> MPYSVGFREADAATSFLRAARSGNLDKALDHLRNGVDINTCNQNGLNGLHLASKEGHVKMVVELLHKEIILETTTKKGNTALHIAALAGQDEVVRELVNYGANVNAQSQKGFTPLYMAAQENHLEVVKFLLENGANQNVATEDGFTPLAVALQQGHENVVAHLINYGTKGKVRLPALHIAARNDDTRTAAVLLQNDPNPDVLSKTGFTPLHIAAHYENLNVAQLLLNRGASVNFTPQNGITPLHIASRRGNVIMVRLLLDRGAQIETKTKDELTPLHCAARNGHVRISEILLDHGAPIQAKTKNGLSPIHMAAQGDHLDCVRLLLQYDAEIDDITLDHLTPLHVAAHCGHHRVAKVLLDKGAKPNSRALNGFTPLHIACKKNHVRVMELLLKTGASIDAVTESGLTPLHVASFMGHLPIVKNLLQRGASPNVSNVKVETPLHMAARAGHTEVAKYLLQNKAKVNAKAKDDQTPLHCAARIGHTNMVKLLLENNANPNLATTAGHTPLHIAAREGHVETVLALLEKEASQACMTKKGFTPLHVAAKYGKVRVAELLLERDAHPNAAGKNGLTPLHVAVHHNNLDIVKLLLPRGGSPHSPAWNGYTPLHIAAKQNQVEVARSLLQYGGSANAESVQGVTPLHLAAQEGHAEMVALLLSKQANGNLGNKSGLTPLHLVAQEGHVPVADVLIKHGVMVDATTRMGYTPLHVASHYGNIKLVKFLLQHQADVNAKTKLGYSPLHQAAQQGHTDIVTLLLKNGASPNEVSSDGTTPLAIAKRLGYISVTDVLKVVTDETSFVLVSDKHRMSFPETVDEILDVSEDEGEELISFKAERRDSRDVDEEKELLDFVPKLDQVVESPAIPRIPCAMPETVVIRSEEQEQASKEYDEDSLIPSSPATETSDNISPVASPVHTGFLVSFMVDARGGSMRGSRHNGLRVVIPPRTCAAPTRITCRLVKPQKLSTPPPLAEEEGLASRIIALGPTGAQFLSPVIVEIPHFASHGRGDRELVVLRSENGSVWKEHRSRYGESYLDQILNGMDEELGSLEELEKKRVCRIITTDFPLYFVIMSRLCQDYDTIGPEGGSLKSKLVPLVQATFPENAVTKRVKLALQAQPVPDELVTKLLGNQATFSPIVTVEPRRRKFHRPIGLRIPLPPSWTDNPRDSGEGDTTSLRLLCSVIGGTDQAQWEDITGTTKLVYANECANFTTNVSARFWLSDCPRTAEAVNFATLLYKELTAVPYMAKFVIFAKMNDPREGRLRCYCMTDDKVDKTLEQHENFVEVARSRDIEVLEGMSLFAELSGNLVPVKKAAQQRSFHFQSFRENRLAMPVKVRDSSREPGGSLSFLRKAMKYEDTQHILCHLNITMPPCAKGSGAEDRRRTPTPLALRYSILSESTPGSLSGTEQAEMKMAVISEHLGLSWAELARELQFSVEDINRIRVENPNSLLEQSVALLNLWVIREGQNANMENLYTALQSIDRGEIVNMLEGSGRQSRNLKPDRRHTDRDYSLSPSQMNGYSSLQDELLSPASLGCALSSPLRADQYWNEVAVLDAIPLAATEHDTMLEMSDMQVWSAGLTPSLVTAEDSSLECSKAEDSDATGHEWKLEGALSEEPRGPELGSLELVEDDTVDSDATNGLIDLLEQEEGQRSEEKLPGSKRQDDATGAGQDSENEVSLVSGHQRGQARITHSPTVSQVTERSQDRLQDWDADGSIVSYLQDAAQGSWQEEVTQGPHSFQGTSTMTEGLEPGGSQEYEKVLVSVSEHTWTEQPEAESSQADRDRRQQGQEEQVQEAKNTFTQVVQGNEFQNIPGEQVTEEQFTDEQGNIVTKKIIRKVVRQIDLSSADAAQEHEEVTVEGPLEDPSELEVDIDYFMKHSKDHTSTPNP;> MSSKYPRSVRRCLPLWALTLEAALILLFYFFTHYDASLEDQKGLVASYQVGQDLTVMAALGLGFLTSNFRRHSWSSVAFNLFMLALGVQWAILLDGFLSQFPPGKVVITLFSIRLATMSAMSVLISAGAVLGKVNLAQLVVMVLVEVTALGTLRMVISNIFNTDYHMNLRHFYVFAAYFGLTVAWCLPKPLPKGTEDNDQRATIPSLSAMLGALFLWMFWPSVNSPLLRSPIQRKNAMFNTYYALAVSVVTAISGSSLAHPQRKISMTYVHSAVLAGGVAVGTSCHLIPSPWLAMVLGLVAGLISIGGAKCLPVCCNRVLGIHHISVMHSIFSLLGLLGEITYIVLLVLHTVWNGNGMIGFQVLLSIGELSLAIVIALTSGLLTGLLLNLKIWKAPHVAKYFDDQVFWKFPHLAVGF;>MRFTFPLMAIVLEIAMIVLFGLFVEYETDQTVLEQLNITKPTDMGIFFELYPLFQDVHVMIFVGFGFLMTFLKKYGFSSVGINLLVAALGLQWGTIVQGILQSQGQKFNIGIKNMINADFSAATVLISFGAVLGKTSPTQMLIMTILEIVFFAHNEYLVSEIFKASDIGASMTIHAFGAYFGLAVAGILYRSGLRKGHENEESAYYSDLFAMIGTLFLWMFWPSFNSAIAEPGDKQCRAIVNTYFSLAACVLTAFAFSSLVEHRGKLNMVHIQNATLAGGVAVGTCADMAIHPFGSMIIGSIAGMVSVLGYKFLTPLFTTKLRIHDTCGVHNLHGLPGVVGGLAGIVAVAMGASNTSMAMQAAALGSSIGTAVVGGLMTGLIL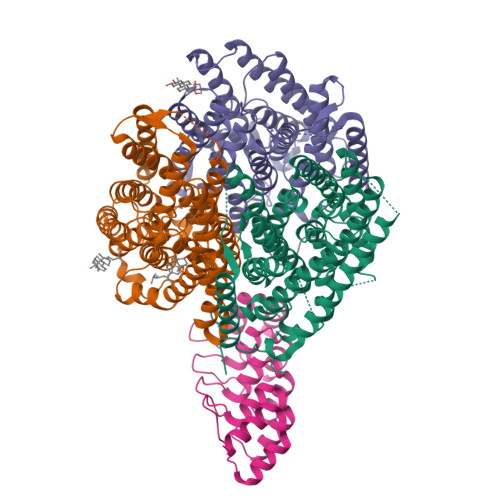KLPLWGQPSDQNCYDDSVYWKVPKTR[2x]>SNPRLTKVLDEMSKKPCVNINEIRKMIRNFQPQFIQPRNGNRPNAQPRTVDSFEWVVRIQSTVETQLLGATNTVPQQTLNLDISFTDDSTTITPASIPGSISMLDNSRHIPAIQSMIQNFKARYLGSLQDTAQLQSPQYPQLLAYLFGQLIAIKDRLDLFRPSNPLSLADALFGFTLAQNARPRYDDHRHAKACQGPLVIPAATNSDCGPCGFVQINANQGLTLPLGACLFVNPETVNDQSFQDFLWLIFATHHRMPNQMQNNWPFSLNIVSTCAAPGRQAPHAGELTDERVRLALDTGHRILLSMFNDDEETLRYYQRKGIETMFRPCCFYTEGGLLRKATRYVSMVPLNGLYYYNGATSYVVSPIHTDAHPGITAAIESFVDIMVLQAVFSFSGPKVVAAKVNASQIDAAMVFGPAVAEGDGFVYDPLRPAPPLSAFYTEFIHRPAEQRIFQMAMSQIYGSHAPLIIANVINSIHNCKTKIVNNKLRATFVRRPPGAPHLKADTAI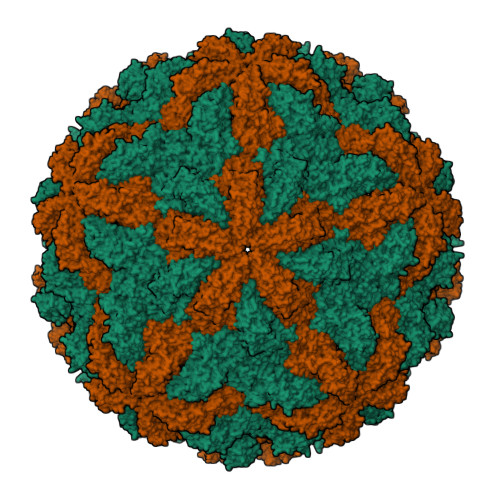INRFHDPELAYALGILADGIAPLDGSHEYNVLDELDYLFNGGDIRNCFGLNALNTRGLGQIVHIRPKREPGKRPRRGFYTTLDGQVHPVTQDAPLDEIYHWRDHGNLTRPYSCHILDSQGLEFADVSNGRSRGKILVVVNSPLKTCAAYQGPSFAPK[2x]> MGQEGKGTCILVGGHEITSGLEVISSLRAIHGLQVEVCPLNGCDYIVSNRMVVERRSQSEMLNSVNKNKFIEQIQHLQSMFERICVIVEKDREKTGDTSRMFRRTKSYDSLLTTLIGAGIRILFSSCQEETADLLKELSLVEQRKNVGIHVPTVVNSNKSEALQFYLSIPNISYITALNMCHQFSSVKRMANSSLQEISMYAQVTHQKAEEIYRYIHYVFD;> MGHIVANEKWRGSQLAQEMQGKIKLIFEDGLTPDFYLSNRCCILYVTEADLVAGNGYRKRLVRVRNSNNLKGIVVVEKTRMSEQYFPALQKFTVLDLGMVLLPVASQMEASCLVIQLVQEQTKEPSKNPLLGKKRALLLSEPSLLRTVQQIPGVGKVKAPLLLQKFPSIQQLSNASIGELEQVVGQAVAQQIHAFFTQPRLEHHHHHH

FANCM is a key component of the FA core complex, which contains a DEAH helicase domain at the N-terminus and a putative nuclease domain and a tandem helix-hairpin-helix (HhH)2 motif domain at the C-terminus. FANCM can interact with the FANCM-associated histone-fold proteins 1 and 2 (MHF1-MHF2) complex via the region following the helicase domain (residues 661–800) and with FAAP24 via the C-terminal domains to form two stable complexes to bind different DNA substrates, which are crucial for FANCM to facilitate repair of ICLs. The FANCM-FAAP24 complex binds preferentially to single-stranded DNA (ssDNA). It plays a key role in the recruitment of the FA core complex to damaged DNA and the monoubiquitylation of FANCD2 (5,18).

We then constructed a slightly shorter form of FANCM (residues 1813–2031, FANCMS) and an N-terminal truncated form of FAAP24 (residues 17–215, FAAP24S), and the resultant FANCMS-FAAP24S complex led to successful crystallization and structure determination of the complex. The crystal structure of the FANCM-FAAP24 complex was solved using the multi-wavelength anomalous dispersion method and refined to 2.9 Å resolution. There is one FANCM-FAAP24 complex in the asymmetric unit, which contains residues 1815–2030 of FANCM and residues 18–213 of FAAP24 except that three solvent-exposed loops (residues 1903–1915 and 1965–1969 of FANCM and residues 147–152 of FAAP24) are disordered. However, the relative position and orientation of the two domains are significantly different: the nuclease domain of FANCM is sandwiched between and interacts with the (HhH)2 domain of FANCM and the nuclease domain of FAAP24, whereas the nuclease domain of FAAP24 is far apart from and has no interaction with the (HhH)2 domain of FAAP24. The two nuclease domains and the two (HhH)2 domains form two compact heterodimers, respectively. The structure of the FANCM-FAAP24 heterodimer has the highest similarity to that of the ApXPF homodimer, even though they share ∼25% sequence identity. Nevertheless, no metal ion is found at the active site of FANCM, despite the fact that there is 2 mM MgCl2 in the protein buffer solution. Taken together, we suggest that the variation of two key residues at the active site and the lack of DNA binding ability of the surrounding region render a catalytically inactive nuclease domain of FANCM and account for the lack of nuclease activity of FANCM-FAAP24. Our structural and functional data together indicate that region II (helix α5′ and the α5′-α6′ loop) of FAAP24 plays a critical role in DNA binding and is essential for the localization of FANCM-FAAP24 to chromatin.6-BROMO-7-[4-(4-CHLOROBENZYL)PIPERAZIN-1-YL]-2-[4-(MORPHOLIN-4-YLMETHYL)PHENYL]-3H-IMIDAZO[4,5-B]PYRIDINE 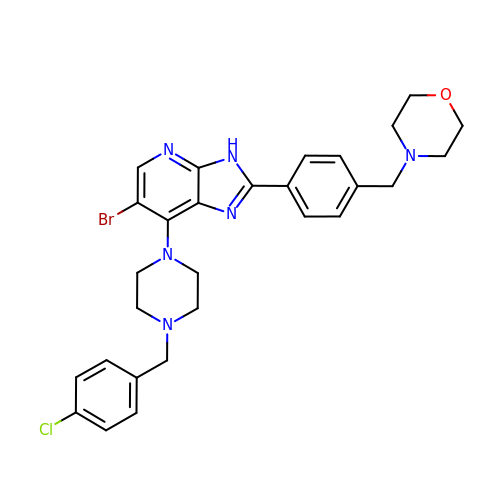| C28 H30 Br Cl N6 O | IZRXRZKKTJHSGV-UHFFFAOYSA-N>SNAMTITNSKAEAWELIGNQFWTIGRVAARPSDRENDIFLENIVPGSTVAVIGASTRFLIEKALERGASVTVFDFSQ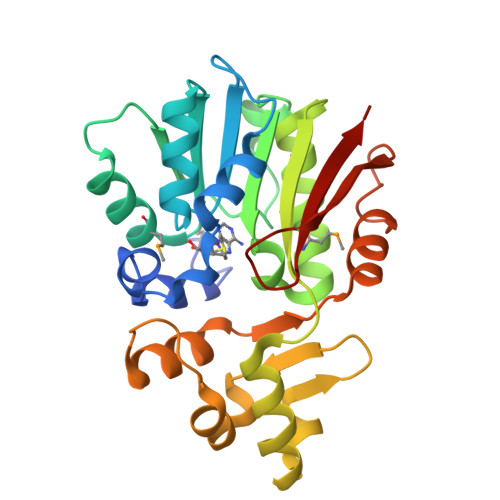RMCDDLAEALADRCVTIDLLDITAEIPKELAGHFDFVLNDRLINRFTTEEARRACLGMLSLVGSGTVRASVKLGFYDIDLKLIEYGEQSGTLAKFFDPSDKTFHFREAGDVLDRALVPHGLIDKPTLLEWYRRRGKETRFDDEDVRALLSHDVVNARGYVTLEKAVELPDAPNTMLYQFSRRAG[4x]>GHMIETIAHPVHEKESAPAGRKMDIVIRAAWQLFLEQGFSATSMDAIAKAAGVSKATLYAYFPSKEALFASLIVAECESLQRDLPVPKLSAGLSEALRDFARQYLHTFIHRKDVAFVRIIANESGRFPVLARLFYESGPEATI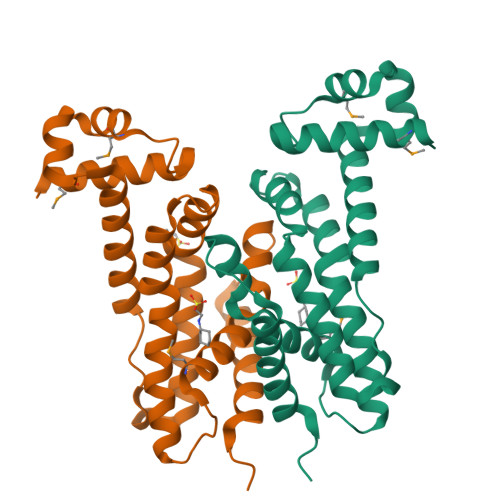RRLAQFLEEARAARVLEFDDPMEAANQFLSLVRGELPLLIVLGLSDLTEEAIEQEIEAGLKFFLKACQPRA[4x]> AMKRAVITGLGIVSSIGNNQQEVLASLREGRSGITFSQELKDSGMRSHVWGNVKLDTTGLIDRKVVRFMSDASIYAFLSMEQAIADAGLSPEAYQNNPRVGLIAGSGGGSPRFQVFGADAMRGPRGLKAVGPYVVTKAMASGVSACLATPFKIHGVNYSISSACATSAHCIGNAVEQIQLGKQDIVFAGGGEELCWEMACEFDAMGALSTKYNDTPEKASRTYDAHRDGFVIAGGGGMVVVEELEHALARGAHIYAEIVGYGATSDGADMVAPSGEGAVRCMKMAMHGVDTPIDYLNSHGTSTPVGDVKELAAI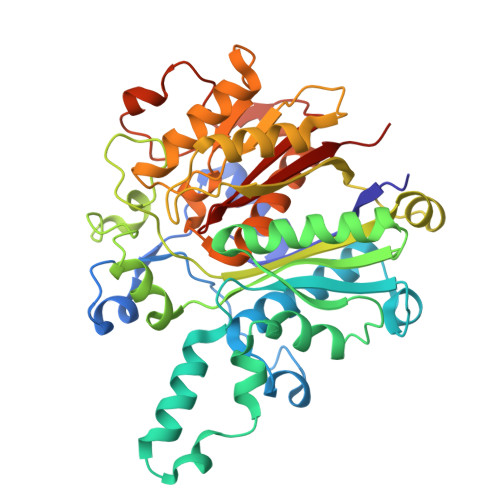REVFGDKSPAISATKAMTGHSLGAAGVQEAIYSLLMLEHGFIAPSINIEELDEQAAGLNIVTETTDRELTTVMSNSFGFGGTNATLVMRKLKD> MLKQVEIFTDGSCLGNPGPGGYGAILRYRGREKTFSAGYTRTTNNRMELMAAIVALEALKE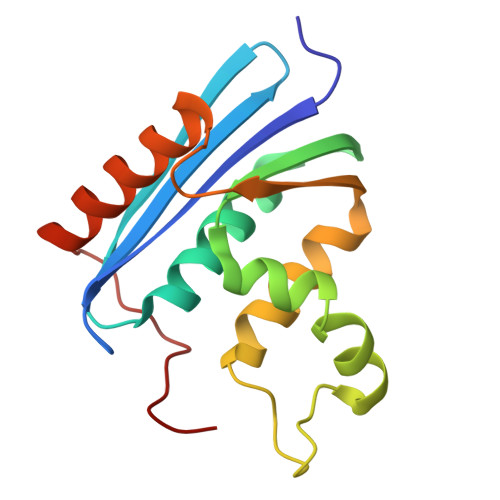HCEVILSTDSQYVRQGITQWIHNWKKRGWKTADAKPVKNVDLWQRLDAALGQHQIKWEWVKGHAGHPENERCDELARAAAMNPTLEDTGYQVEV> MSNDEKEKLKELLKRAEELAKSPDPEDLKEAVRLAEEVVRERPGSEAAKKALEIIQEAAELLKKSPD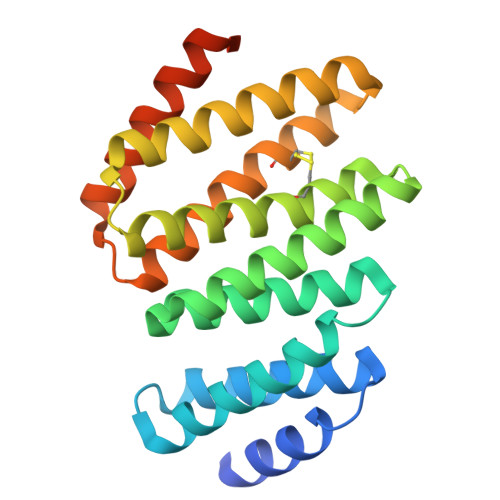PEAIIAAARALLKIAATTGDNEAAKQAIEAASKAAQLAEQRGDDELVCEALALLIAAQVLLLKQQGTSDEEVAEHVARTISQLVQRLKRKGASYEVIKECVQRIVEEIVEALKRSGTSEDEINEIVRRVKSEVERTLKESGSSGWLEHHHHHH beta-methylnorleucine 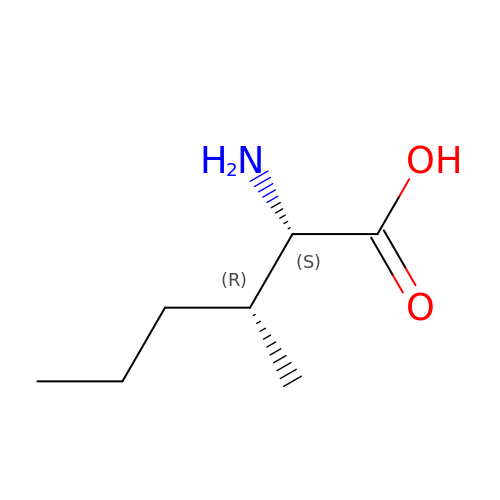| C7 H15 N O2 | KWSUGULOZFMUDH-RITPCOANSA-N> MRGSHHHHHHGSSYQIAVLAGDGIGPEVMAEARKVLKAVEARFGLNIEYTEYDVGGIAIDNHGCPLPEATLKGCEAADAILFGSVGGPKWEKLPPNEQPERGALLPLRGHFELFCNLRPAKLHDGLEHMSPLRSDISARGFDVLCVRELTGGIYFGKPKGRQGEGESEEAFDTMRYSRREISRIARIAFEAARGRRKKVTSVDKANVLACS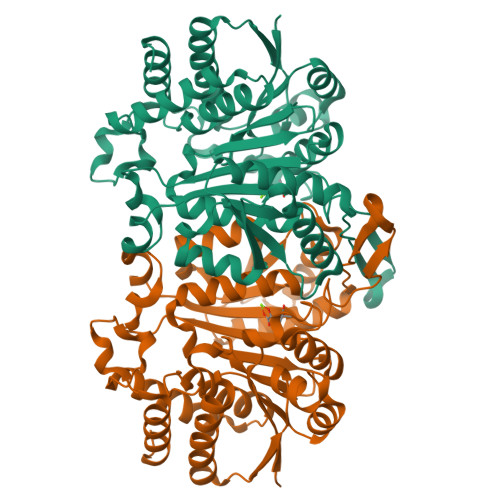VLWRQVVEEVAVDFPDVELEHIYIDNATMQLLRRPDEFDVMLCSNLFGDILSDEIAMLTGSMGLLASASMNSTGFGLFEPAGGSAPDIAGKGIANPIAQILSAALMLRHSLKQEEAASAIERAVTKALNSGYLTGELLSSDQRHKAKTTVQMGDFIADAVKAGV> PLHSIISSTESVQGSTSKHEFQAETKKL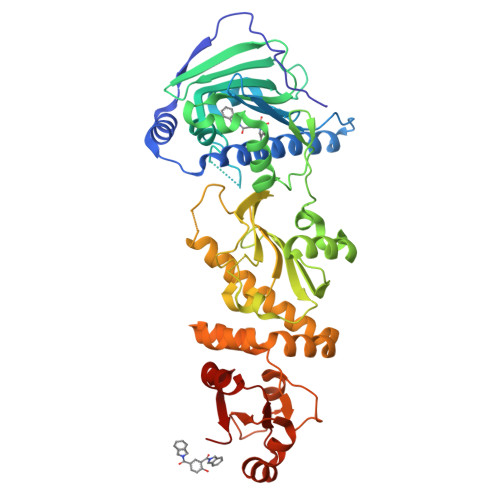LDIVARSLYSEKEVFIRELISNASDALEKLRHKLVSDGQALPEMEIHLQTNAEKGTITIQDTGIGMTQEELVSNLGTIARSGSKAFLDALQNQAEASSKIIGQFGVGFYSAFMVADRVEVYSRSAAPGSLGYQWLSDGSGVFEIAEASGVRTGTKIIIHLKSDCKEFSSEARVRDVVTKYSNFVSFPLYLNGRRMNTLQAIWMMDPKDVREWQHEEFYRYVAQAHDKPRYTLHYKTDAPLNIRSIFYVPDMKPSMFDVSRELGSSVALYSRKVLIQTKATDILPKWLRFIRGVVDSEDIPLNLSRELLQESALIRKLRDVLQQRLIKFFIDQSKKDAEKYAKFFEDYGLFMREGIVTATEQEVKEDIAKLLRYESSALPSGQLTSLSEYASRMRAGTRNIYYLCAPNRHLAEHSPYYEAMKKKDTEVLFCFEQFDELTLLHLREFDKKKLISVET> MTNIFTPIEEALEAYKNGEFLIVMDDEDRENEGDLIMAAELITQEKMAFL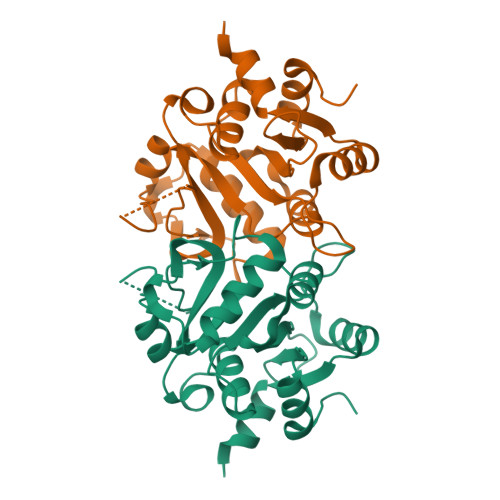VRYSSGYVCVPLSEERANQLELPPMLANRSDRHGTAYTITCDFAEGTTTGISAHDRALTTRSLANPNSKPQDFIKPGHILPLRAVPGLLKKRRGHTEAAVQLSTLAGLQPAGVICELVRDEDGLMMRLDDCIQFGKKHGIKIININQLVEYISK>MTGDHIKVIFFNGRGRAESIRMTLVAAGVNYEDERISFQDWPKIKPTIPGGRLPAVKITDNHGHVKWMVESLAIARYMAKKHHMMGGTEEEYYNVEKLIGQAEDLEHEYYKTLMKPEEEKQKIIKEILNGKVPVLLDIICESLKASTGKL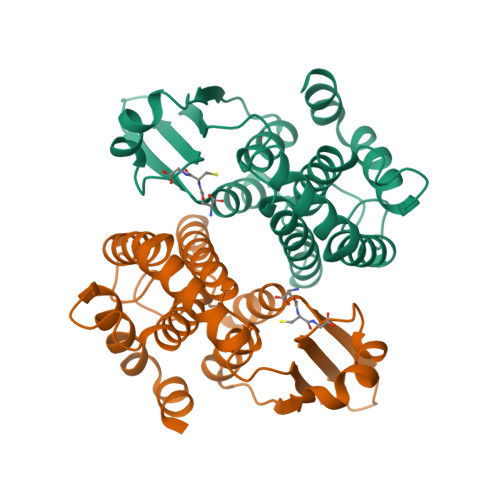AVGDKVTLADLVLIAVIDHVTDLDKEFLTGKYPEIHKHRENLLASSPRLAKYLSDRAATPF[2x]>MEYKVTPPAVLREPLVTPNKLL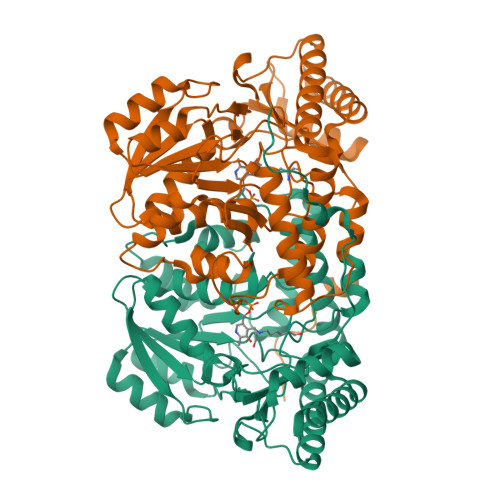MGPGPSNAPQRVLDAMSRPILGHLHPETLKIMDDIKEGVRYLFQTNNIATFCLSASGHGGMEATLCNLLEDGDVILIGHTGHWGDRSADMATRYGADVRVVKSKVGQSLSLDEIRDALLIHKPSVLFLTQGDSSTGVLQGLEGVGALCHQHNCLLIVDTVASLGGAPMFMDRWEIDAMYTGSQKVLGAPPGITPVSFSHRAVERYKRRNTKVKVYYWDMSLVGDYWGCFGRPRIYHHTISSTLLYGLREAIAMACEEGLPALIARHEDCAKRLYRGLQDAGFELYADPKDRLSTVTTIKVPQGVDWLKAAQYAMKTYLVEISGGLGPTAGQVFRIGLMGQNATTERVDRVLQVFQEAVAAVKPDVQVKGKM[2x]> GKEFWNLDKNLQLRLGIVFLGAFSYGTVFSSMTIYYNQYLGSAITGILLALSAVATFVAGILAGFFADRNGRKPVMVFGTIIQLLGAALAIASNLPGHVNPWSTFIAFLLISFGYNFVITAGNAMIIDASNAENRKVVFMLDYWAQNLSVILGAALGAWLFRPAFEALLVILLLTVLVSFFLTTFVMTETFKPTVKVDNIFQAYKTVLQDKTYMIFMGANIATTFIIMQFDNFLPVHLSNSFKTITFWGFEIYGQRMLTIYLILACVLVVLLMTTLNRLTKDWSHQKGFIWGSLFMAIGMIFSFLTTTFTPIFIAGIVYTLGEIVYTPSVQTLGADLMNPEKIGSYNGV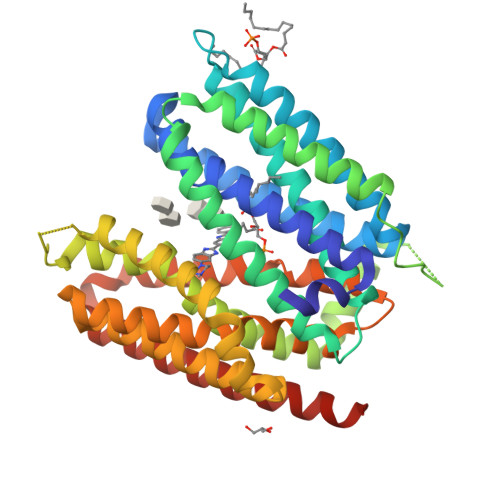AAIKMPIASILAGLLVSISPMIKAIGVSLVLALTEVLAIILVLVAVNRHQKTKLNLEVLFQG>MVKQIESKTAFQEALDAAGDKLVVVDFSATWCGPCKMIKPFFHSLSEKYSNVIFLEVDVDDCQDVASECEVKCMPTFQFFKKGQKVGEFSGANK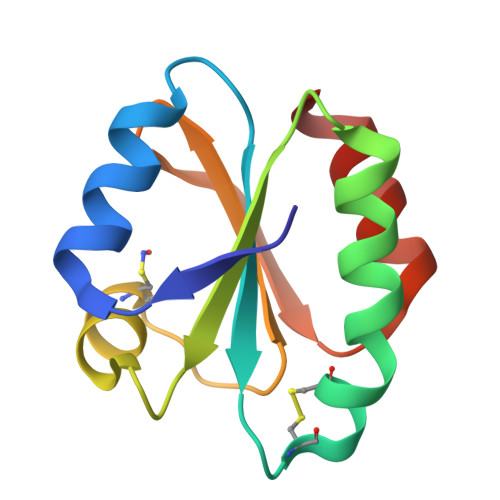EKLEATINELV[3x]>TRDQNGTWEMESNENFEGYMKALDIDFCTRKIAVRCTQTKVIDQDGDNFKDKTTSTFHHHHHHRNYDVDFTVGVEFDEYTKSLDNRHVKALVTWEGDVLVCVQKGEKKNRG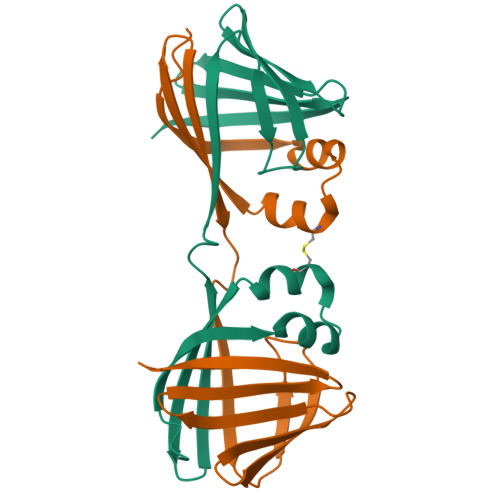WKKWIEGDKLYLELTCGDQVCRQVFKKK[2x]>[3x]MNSICSLYCLFRRVMPYSSEILSSTVYRPPFLATSGLFFTRDHYKFIIMNQQQINPAQRSLRPRAQSAPSRSARRRRNRRRRNPSTPAGTVALQPSRITRRVVSNLARRPLTITTAGLAWLRQYLNPMGPSTSSVSGFPDGSAVTTCIADYTNTFNISFPPREAIYCTGSNSDEKPVMLDAATYAKIDAWTKSDITLCILALPMLRNVVMIRLYASTPTAFTLSEGVPNFVQRFPNWSAFTTEGKVLNNGDSPGYIQSFVYLPNVDKHLSAARGFRLLSRGLTGIYTAPSLETQGFVTACQYLAEGALQTQTVGNDFVQSVEVNADKTVKNVNGKRLHYSGPPKFVFPLEGDNCAPSSLVETYHQAYQARAVDGFYMPILSSSRDNPFISPKPQPIAVFNRWYYRGCLDPVPASKVADGPSQYYYDLNVADDVAPLYNTGVVWMEGISSKFSLKLKTRTVIQYIPTSGSVLANFTRHEPTYDQVALDAADRIRNMMPHAYPAAYNDWGWLGDLLDSTLSMLPGIGTAYRFAKPLIKPAWNWLGGKVSDFFGNPVSRDGDIYFDAK

The RNA genome sizes of LSV1 and LSV2 are ~5.6 kb, encoding three major genes: the Orf1 with the unclear function, RdRP responsible for viral RNA replication, and the capsid protein (CP) for the host recognition and viral capsid assembly. CP forms the capsid shell that protects genomes and is responsible for both host specificity and receptor binding to transport the viral genome into infected host cells, or for intracellular trafficking. We determine cryo-EM structures of T = 4 and T = 3 capsids of virus-like particles (VLPs) of Lake Sinai virus (LSV) 2 and delta-N48 LSV1, belonging to tetraviruses, at resolutions of 2.3–2.6 Å in various pH environments. Analyses of these capsid structures reveal the intermolecular interactions that drive subunits assembly into homo-trimeric capsomeres and eventually into a complete viral capsid in which specific domains, such as the N-terminal domain, the helical domain, and the β-barrel domain/C-arm, could encapsidate nucleic acids.

To investigate the positions of sequence variations in the context of the VLP, we truncated the extra N-terminal 48 residues of LSV1 CP, namely delta-N48 LSV1 CP, which self-assembled in vitro into delta-N48 LSV1 VLP, for cryo-EM structural analysis to inspect the structural differences at the regions of low sequence homology. We reconstructed the density maps of the T = 4 and T = 3 delta-N48 LSV1 VLPs at 4.8 and 3.5 Å resolution, respectively, by gold-standard (0.143) FSC. We could only determine the structure of the T = 3 delta-N48 LSV1 VLP because the densities of several large side chains were apparent and the rotamers could be properly modeled. The cryo-EM structure of the T = 3 delta-N48 LSV1 VLP comprises residues 96−558 of subunits A, B, and C, in which residues 49–95 of NTD with N-ARM and the last residues 559–565 of CTD are disordered. The helical domain of T = 3 delta-N48 LSV1 CP comprises a three-helix fold as found in LSV2 CP, but is equipped with an additional N-terminal distal helix (α1’, residues 96–104) that associates with the core (α1, α11, and α12) of the helical domain. Delta-N48 LSV1 CP interacts with ssRNA via the rigid helix α1’, α1’–α1 loop, β-barrel domain, and C-arm. In addition, the focused refinement reconstruction in T = 3 delta-N48 LSV1 VLP further shows a visualization of the RNA coordination, in which a two-based single-strand RNA (ssRNA) was partially resolved. K545 and R556 are two basic residues on the C-arm, but only the side chain of R556 faces the ssRNA-binding site, as does that of R370. This ssRNA-binding site is formed by the dynamic C-arm and the βF–βG loop of the central β-barrel domain.The enzyme 15-prostaglandin dehydrogenase (15-PGDH) is a key negative regulator of tissue stem cell activity in proliferation and in the repair of tissue injury, whose negative regulation of tissue regeneration is conserved across multiple organs. 15-PGDH acts via its NAD+-dependent enzymatic activity of oxidizing and degrading prostaglandin E2 (PGE2), and related eicosanoids, which provide key trophic support for stem cells in multiple tissues. Specifically, 15-PGDH catalyzes the rate-limiting step to initiate PGE2 degradation by oxidizing the 15-hydroxyl moiety of PGE2 to a 15-keto group, thereby inactivating PGE2 from being able to bind to its receptors. 15-PGDH assembled as a homodimer, which is the proposed physiological form of the enzyme.

To further define the predicted functional role of the 15-PGDH drug binding lid, we employed cryo-EM to solve the structure of the 15-PGDH-NADH complex in the absence of inhibitor. With a similar imaging processing workflow, we were able to resolve the apo-form to 3.3 Å. The cryo-EM map of the unliganded 15-PGDH shows clear differences from the (+)-SW209415-bound complex described above. In the absence of inhibitor, 15-PGDH forms a looser complex that lacks certain structural features because of enhanced dynamic flexibility. These features are apparent in the 2D class averages and localize mainly to the lid region of the inhibitor binding pocket. Thus, the MD simulations recapitulate the cryo-EM findings that the lid becomes disordered in the absence of inhibitor binding. In the absence of an inhibitor, our data indicate that this lid of 15-PGDH successively swings between open-and-closed states in solution.

>MHVNGKVALVTGAAQGIGRAFAEALLLKGAKVALVDWNLEAGVQCKAALDEQFEPQKTLFIQCDVADQQQLRDTFRKVVDHFGRLDILVNNAGVNNEKNWEKTLQINLVSVISGTYLGLDYMSKQNGGEGGIIINMSSLAGLMPVAQQPVYCASKHGIVGFTRSAALAANLMNSGVRLNAICPGFVNTAILESIEKEENMGQYIEYKDHIKDMIKYYGILDPPLIANGLITLIEDDALNGAIMKITTSKGIHFQDY[2x]> GSHMVTTIPFWHSMEGELGKEVDSLAQRFNAENPDYKIVPTYKGNYEQNLSAGIAAFRTGNAPAILQVYEVGTATMMASKAIKPVYDVFKEAGIQFDESQFVPTVSGYYSDSKTGHLLSQPFNSSTPVLYYNKDAFKKAGLDPEQPPKTWQDLADYAAKLKASGMKCGYASGWQGWIQLENFSAWNGLPFASKNNGFDGTDAVLEFNKPEQVKHIAMLEEMNKKGDFSYVGRKDESTEKFYNGDCAMTTASSGSLANIREYAKFNYGVGMMPYDADAKDAPQNAIIGGASLWVMQGKDKETYTGVAKFLDFLAKPENAAEWHQKTGYLPITKAAYDLTREQGFYEKNPGADTATRQMLNKPPL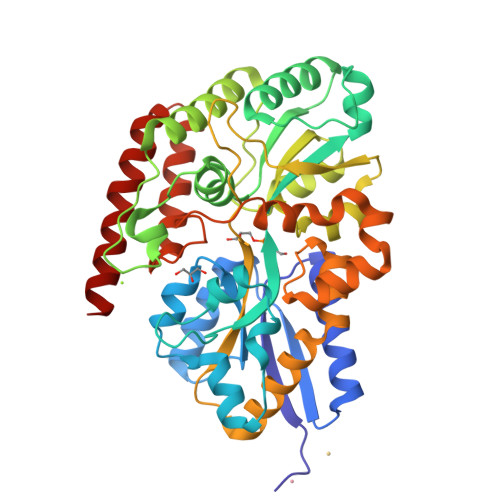PFTKGLRLGNMPQIRVIVDEELESVWTGKKTPQQALDTAVERGNQLLRRFEKSTKS> PPAQLSVHTVSWNSGHERAPTNLEELLGLNSGETPDVIAVAVQGFGFQTDKPQQGPACVKNVQSLLTSKGYTKLKNTITETMGLTVYCLEKHLDQNTLKNETIIVTVDDQKKSGGIVTSFTIYNKRFSFTTSRMSDEDVTSTNTKYAYDTRLDYSKKDDPSDFLFWIGDLNVRVETNATHAKSLVDQNNIDGLMAFDQLKKAKEQKLFDGWTEPQVTFKPTYKFKPNTDEYDLSATPSWTDRALYKSGTGKTIQPLSYNSLTNYKQTEHRPV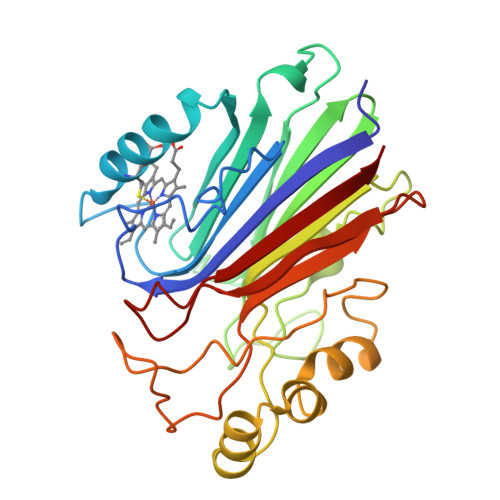LAKFRVTL> IVGGYTCQENSVPYQVSLNSGYHFCGGSLINDQWVVSAAHCYKSRIQVRLGEHNINVLEGNEQFVNAAKIIKHPNFDRETYNNDIMLIKLSSPVKLNARVATVALPSSCAPAGTQCLISGWGNTLSSGVNEPDLLQCLDAPLLPQADCEASSSFIITDNMVCVGFLEGGKDACQGDSGGPVVCNGELQGIVSWGYGCALPDNPGVYTKVCN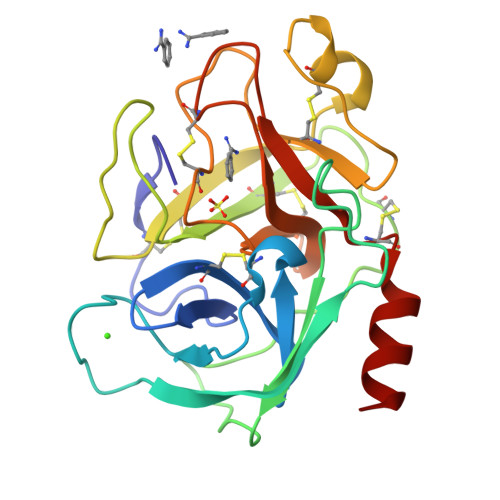YVDWIQDTIAAN>PQPPADEQPEPRTRRRAYLWCKEFLPGAWRGLREDEFHISVIRGGLSNMLFQCSLPDTTATLGDEPRKVLLRLYGAILQMRSCNKEGSEQAQKENEFQGAEAMVLESVMFAILAERSLGPKLYGIFPQGRLEQFIPSRRLDTEELSLPDISAEIAEKMATFHGMKMPFNKEPKWLFGTMEKYLKEVLRIKFTEESRIKKLHKLLSYNLPLELENLRSLLESTPSPVVFCHNDCQEGNILLLEGRENSEKQKLMLIDFEYSSYNYRGFDIGNHFCEWMYDYSYEKYPFFRANIRKYPTKKQQLHFISSYLPAFQNDFENLSTEEKSIIKEEMLLEV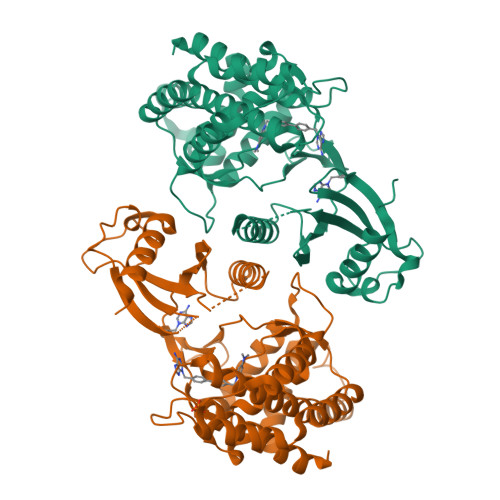NRFALASHFLWGLWSIVQAKISSIEFGYMDYAQARFDAYFHQKRKLGV[2x]> GSTEGKGSGLQGHIIENPQYFSDACVHHIKRRDIVLKWELGEGAFGKVFLAECHNLLPEQDKMLVAVKALKEASESARQDFQREAELLTMLQHQHIVRFFGVCTEGRPLLMVFEYMRHGDLNRFLRSHGPDAKLLAGGEDVAPG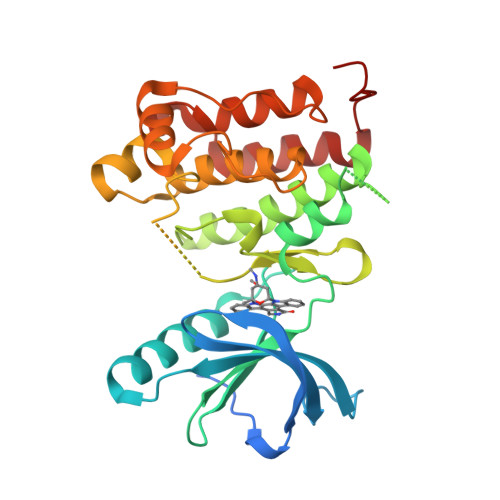PLGLGQLLAVASQVAAGMVYLAGLHFVHRDLATRNCLVGQGLVVKIGDFGMSRDIYSTDYYRVGGRTMLPIRWMPPESILYRKFTTESDVWSFGVVLWEIFTYGKQPWYQLSNTEAIDCITQGRELERPRACPPEVYAIMRGCWQREPQQRHSIKDVHARLQALAQAPPVYLDVLG> MNNDKRGLNVELSKEISKRVVEHRNRFKRLMFNRYLEFLPLLINYTNRDTVGIDFIQLESALRQNINVVVGEARNKQIMILGYVNNTYFNQAPNFSSNFNFQFQKRLTKEDIYFIVPDYLIPDDCLQIHKLYDNCMSGNFVVMQNKPIQYNSDIEIIEHYTDELAEVALSRFSLIMQAKFSKIFKSEINDESINQLVSEIYNGAPFVKMSPMFNADDDIIDLTSNSVIPALTEMKREYQNKISELSNYLGINSLAVDKESGVSDEEAKSNRGFTTSNSNIYLKGREPITFLSKRYGLDIKPYYDDETTSKISMVDTLFKDESSDING;> MARYTMTLYDFIKSELIKKGFNEFVNDNKLTFYDDEFQFMQKMLKFDKDVLAIVNEKVFKGFSLKDELSDLLFKKSFTIHFLDREINRQTVEAFGMQVITVCITHEDYLNVVYSSSEVEKYLQSQGFTEHNEDTTSNTDETSNQNATSLDNSTGMTANRNAYVSLPQSEVNIDVDNTTLRFADNNTIDNGKTVNKSSNESNQNAKRNQNQKGNAKGTQFTKQYLIDNIDKAYDLRKKILNEFDKKCFLQIW;>[3x]MAYNENDFKYFDDIRPFLDEIYKTRERYTPFYDDRADYNTNSKSYYDYISRLSKLIEVLARRIWDYDNELKKRFKNWDDLMKAFPEQAKDLFRGWLNDGTIDSIIHDEFKKYSAGLTSAFALFKVTEMKQMNDFKSEVKDLIKDIDRFVNGFELNELEPKFVMGFGGIRNAVNQSINIDKETNHMYSTQSDSQKPEGFWINKLTPSGDLISSMRIVQGGHGTTIGLERQSNGEMKIWLHHDGVAKLLQVAYKDNYVLDLEEAKGLTDYTPQSLLNKHTFTPLIDEANDKLILRFGDGTIQVRSRADVKNHIDNVEKEMTIDNSENNDNRWMQGIAVDGDDLYWLSGNSSVNSHVQIGKYSLTTGQKIYDYPFKLSYQDGINFPRDNFKEPEGICIYTNPKTKRKSLLLAMTNGGGGKRFHNLYGFFQL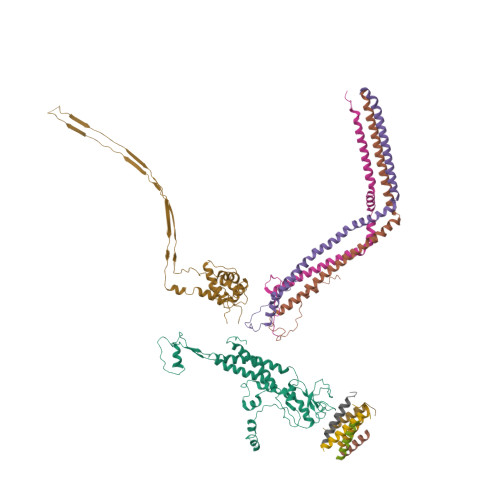GEYEHFEALRARGSQNYKLTKDDGRALSIPDHIDDLNDLTQAGFYYIDGGTAEKLKNMPMNGSKRIIDAGCFINVYPTTQTLGTVQELTRFSTGRKMVKMVRGMTLDVFTLKWDYGLWTTIKTDAPYQEYLEASQYNNWIAYVTTAGEYYITGNQMELFRDAPEEIKKVGAWLRVSSGNAVGEVRQTLEANISEYKEFFSNVNAETKHREYGWVAKHQK;>[6x]MTEFDEIVKPDDKEETSESTEENLESTEETSESTEESTEESTEESTEDKTVETIEEENENKLEPTTTDEDSSKFDPVVLEQRIASLEQQVTTFLSSQMQQPQQVQQTQSDVTESNKEDNDYSDEELVDKLDLD>SRIFYLRNFNNWMKSVLIGEFLEKVRQKKKRDITVLDLGCGKGGDLLKWKKGRINKLVCTDIADVSVKQCQQRYEDMKNRRDSEYIFSAEFITADSSKELLIDKFRDPQMCFDICSCQFVCHYSFESYEQADMMLRNACERLSPGGYFIGTTPNSFELIRR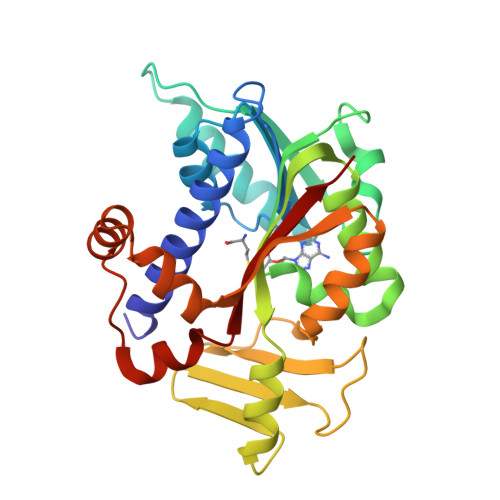LEASETESFGNEIYTVKFQKKGDYPLFGCKYDFNLEGVVDVPEFLVYFPLLNEMAKKYNMKLVYKKTFLEFYEEKIKNNENKMLLKRMQGGSGSKSEWEATSIYLVFAFEKQQ[2x]>MGVFDRIRGALGRGLDVFRGDLPQVQPPAPQPAPAPAIT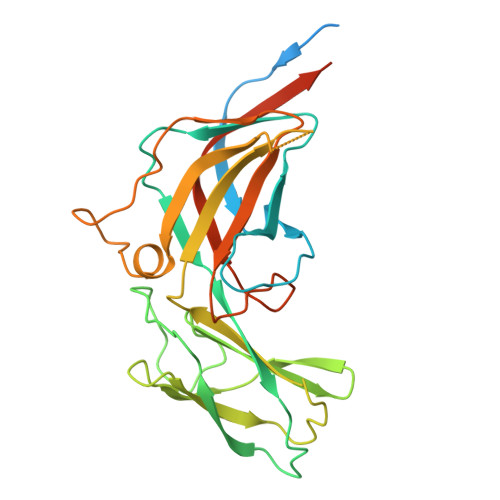PAAVQVGGWGFAWIDNEDFSPTGLAWRSGEYFALAQMKTPETAHFRIAAQERRLRIYLRGQKVVNGRNLSDPDSRTVNLPFLMQTPQGAPTLPSTYHPDVAVWAKVGSTWQPCVITAINYSTGDVTFTEPAGVTASDGIEIYYVHGDGQFRLRVARDAGGVDDSAATVFNQSFSTMHSVDQNNVETMIAWPQQVELVPGTRLVLEVFTTQVPMVWNERSGHYIQIAAMGRRIEVLDKGGLQRLAELEARGGL[2x]> KDSSDEASVSPIADNEREAVTLLLGYLEDKDQLDFYSGGPLKALTTLVYSDNLNLQRSAALAFAEITEKYVRQVSREVLEPILILLQSQDPQIQVAACAALGNLAVNNENKLLIVEMGGLEPLINQMMGDNVEVQCNAVGCITNLATRDDNKHKIATSGALIPLTKLAKSKHIRVQRNATGALLNMTHSE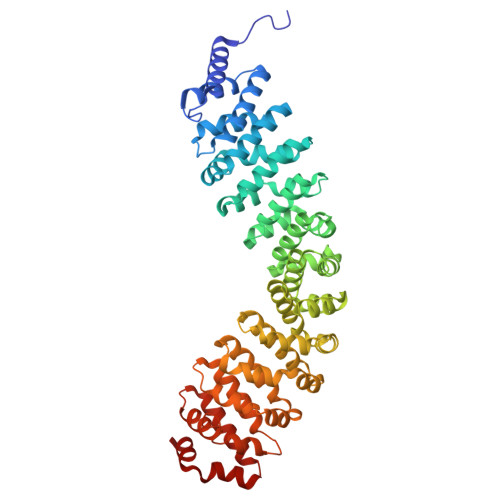ENRKELVNAGAVPVLVSLLSSTDPDVQYYCTTALSNIAVDEANRKKLAQTEPRLVSKLVSLMDSPSSRVKCQATLALRNLASDTSYQLEIVRAGGLPHLVKLIQSDSIPLVLASVACIRNISIHPLNEGLIVDAGFLKPLVRLLDYKDSEEIQCHAVSTLRNLAASSEKNRKEFFESGAVEKCKELALDSPVSVQSEISACFAILALADVSKLDLLEANILDALIPMTFSQNQEVSGNAAAALANLCSRVNNYTKIIEAWDRPNEGIRGFLIRFLKSDYATFEHIALWTILQLLESHNDKVEDLVKNDDDIINGVRK>[2x]MLNLKVGIIGAGPSGLAMLRAFESEQKKGNPIPEIKCYEKQDNWGGMWNYTWRTGVGKYGEPIHGSMYK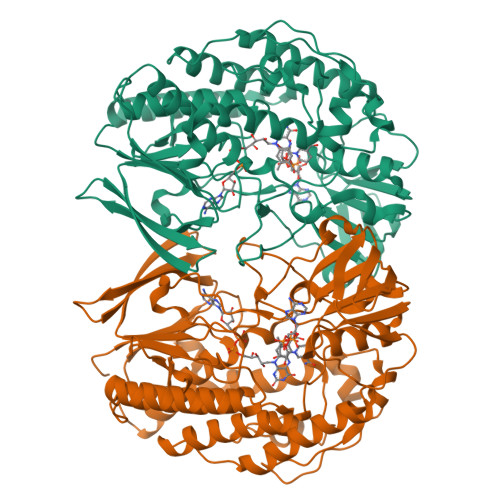YLWSNGPKECLEFSDYTFMEHFKQPISSYPPREVLFDYIQGRIKQSNARDFIKFNTVARWVDYLEDKKQFRVIFDDLVKNETFEEYFDYLVVGTGHFSTPNMPYFKGIDSFPGTVMHAHDFRGADQFIDKDILLIGSSYSAEDIGVQCFKHGSKSVTISYRTNPIGAKWPKGIEEKPIVTHFEDNVAHFKDGSKKEYDAVILCTGYQHKFPFLPDNLRLKTKNNLYPDNLYKGVVFNENERLIFLGMQDQYYTFNMFDTQAWFARDYMLGRIALPNKEIRDKDIAKWVELEKTSVTGEEHVDFQTDYIKELIEMTDYPTFDLDRVAEMFKSWLNDKETNILNYRDKVYTSVMTGVTAEEHHTPWMKELDDSLERYLDEVEVDELELSKENYYHHHHHH> MENLNHCPLEDIKVNPWKTPQSTARVITLRVEDPNEINNLLSINEIDNPNYILQAIMLANAFQNALVPTSTDFGDALRFSMPKGLEIANTITPMGAVVSYVDQNVTQTNNQVSVMINKVLEVLKTVLGVALSGSVIDQLTAAVTNTFTNLNTQKNEAWIFWGKETANQTNYTYNVLFAIQNAQTGGVMYCVPVGFEIKVSAVKEQVLFFTIQDSASYNVNIQSLKFAQPLVSSSQYPIADLTSAINGTL

The active ingredient of Bti is a parasporal body that contains three natural sub-micron-sized crystals of four highly efficient mosquito-specific toxins, namely Cyt1Aa, Cry11Aa and co-crystallizing Cry4Aa and Cry4Ba. Following ingestion by mosquito larvae, the crystals promptly dissolve in the alkaline environment of the gut (pH ~11), releasing protoxins that are activated into toxins through proteolytic cleavage of propeptides by gut enzymes. Each activated protein eventually self-assembles into cytolytic oligomers that perforate gut cells, leading to mosquito larvae death. Here, we use serial femtosecond crystallography (SFX) at an X-ray free electron laser (XFEL) to identify the features governing the in vivo crystallization of Cyt1Aa in Bti cells, and to track the structural dynamics driving natural crystal dissolution in the alkaline mosquito larvae gut.

We produced sub-micron-sized crystals of Cyt1Aa in vivo by recombinant expression in an acrystalliferous strain of Bti (4Q7). Using SFX at the CXI-SC3 micro-focused beamline10 of the Stanford Linear Accelerator Center (SLAC) Linac Coherent Light Source (LCLS), diffraction data extending to 1.86 Å could be collected at room temperature (RT) for the wild-type (WT) Cyt1Aa protoxin at pH 7 (“pH7” dataset), from sub-micron-sized crystals injected by a MESH device. Clear residual density allowed us to build most of these residues (H6-L249). At the monomeric level, the Cyt1Aa protoxin displays a conformation overall similar to that of the activated toxin, with two outer layers of α-helix hairpins, αA/αB and αC/αD, respectively covering the hydrophilic and hydrophobic sides of a central five-stranded mixed β-sheet (namely β2-β5-β6-β7-β3). In vivo-grown Cyt1Aa protoxin crystals are remarkably packed, burying 40.1% of surface area at crystal contacts (5484.2 Å2 out of 13661.2 Å2 of total monomeric areas), compared with only 13.3% (1252.7 Å2 out of 9405.5 Å2) in crystals of the activated toxin grown in vitro. Examination at the unit-cell level reveals that the Cyt1Aa protoxin crystallizes as a domain-swapped (DS) dimer13 with strands β1 (contributed by the N-terminal propeptide) and β2 entwined at the DS interface (interface #1), aligned with a crystallographic two-fold axis. Formation of the DS dimer thus likely precedes crystallization in Bti cells. Strikingly, residues absent from the activated toxin structure are the main contributors to the packing of the natural crystals. Most notably, the N-terminal propeptide buries 73% of its surface area (2704 over 3691 Å2) across nine interaction zones, contributing 34 H-bonds, 10 salt-bridges and a disulfide bridge at position C7. This disulfide bridge is aligned with the other crystallographic two-fold axis.> GAEFMDLDQGGEALAPRQVLDLEDLVFTQGSHFMANKRCQLPDGSFRRQRKGYEEVHVPALKPKPFGSEEQLLPVEKLPKYAQAGFEGFKTLNRIQSKLYRAALETDENLLLCAPTGAGKTNVALMCMLREIGKHINMDGTINVDDFKIIYIAPMRSLVQEMVGSFGKRLATYGITVAELTGDHQLCKEEISATQIIVCTPEKWDIITRKGGERTYTQLVRLIILDEIHLLHDDRGPVLEALVARAIRNIEMTQEDVRLIGLSATLPNYEDVATFLRVDPAKGLFYFDNSFRPVPLEQTYVGITEKKAIKRFQIMN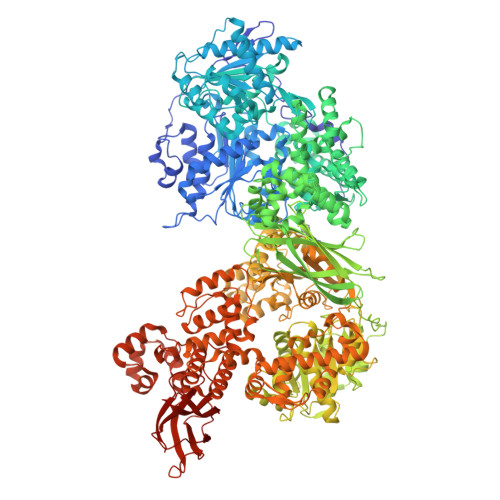EIVYEKIMEHAGKNQVLVFVHSRKETGKTARAIRDMCLEKDTLGLFLREGSASTEVLRTEAEQCKNLELKDLLPYGFAIHHAGMTRVDRTLVEDLFADKHIQVLVSTATLAWGVNLPAHTVIIKGTQVYSPEKGRWTELGALDILQMLGRAGRPQYDTKGEGILITSHGELQYYLSLLNQQLPIESQMVSKLPDMLNAEIVLGNVQNAKDAVNWLGYAYLYIRMLRSPTLYGISHDDLKGDPLLDQRRLDLVHTAALMLDKNNLVKYDKKTGNFQVTELGRIASHYYITNDTVQTYNQLLKPTLSEIELFRVFSLSSEFKNITVREEEKLELQKLLERVPIPVKESIEEPSAKINVLLQAFISQLKLEGFALMADMVYVTQSAGRLMRAIFEIVLNRGWAQLTDKTLNLCKMIDKRMWQSMCPLRQFRKLPEEVVKKIEKKNFPFERLYDLNHNEIGELIRMPKMGKTIHKYVHLFPKLELSVHLQPITRSTLKVELTITPDFQWDEKVHGSSEAFWILVEDVDSEVILHHEYFLLKAKYAQDEHLITFFVPVFEPLPPQYFIRVVSDRWLSCETQLPVSFRHLILPEKYPPPTELLDLQPLPVSALRNSAFESLYQDKFPFFNPIQTQVFNTVYNSDDNVFVGAPTGSGKTICAEFAILRMLLQSSEGRCVYITPMEALAEQVYMDWYEKFQDRLNKKVVLLTGETSTDLKLLGKGNIIISTPEKWDILSRRWKQRKNVQNINLFVVDEVHLIGGENGPVLEVICSRMRYISSQIERPIRIVALSSSLSNAKDVAHWLGCSATSTFNFHPNVRPVPLELHIQGFNISHTQTRLLSMAKPVYHAITKHSPKKPVIVFVPSRKQTRLTAIDILTTCAADIQRQRFLHCTEKDLIPYLEKLSDSTLKETLLNGVGYLHEGLSPMERRLVEQLFSSGAIQVVVASRSLCWGMNVAAHLVIIMDTQYYNGKIHAYVDYPIYDVLQMVGHANRPLQDDEGRCVIMCQGSKKDFFKKFLYEPLPVESHLDHCMHDHFNAEIVTKTIENKQDAVDYLTWTFLYRRMTQNPNYYNLQGISHRHLSDHLSELVEQTLSDLEQSKCISIEDEMDVAPLNLGMIAAYYYINYTTIELFSMSLNAKTKVRGLIEIISNAAEYENIPIRHHEDNLLRQLAQKVPHKLNNPKFNDPHVKTNLLLQAHLSRMQLSAELQSDTEEILSKAIRLIQACVDVLSSNGWLSPALAAMELAQMVTQAMWSKDSYLKQLPHFTSEHIKRCTDKGVESVFDIMEMEDEERNALLQLTDSQIADVARFCNRYPNIELSYEVVDKDSIRSGGPVVVLVQLEREEEVTGPVIAPLFPQKREEGWWVVIGDAKSNSLISIKRLTLQQKAKVKLDFVAPATGAHNYTLYFMSDAYMGCDQEYKFSVDVKEAETDSDSD> XHALYA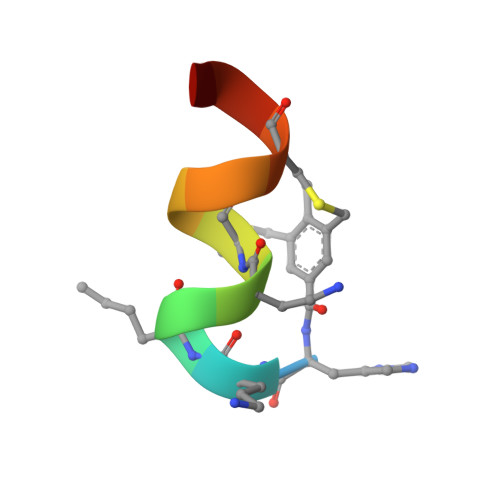CIRCYAX> SSKQKVDLQSLPTRAYLDQTVVPILLQGLAVLAKERPPNPIEFLASYLLK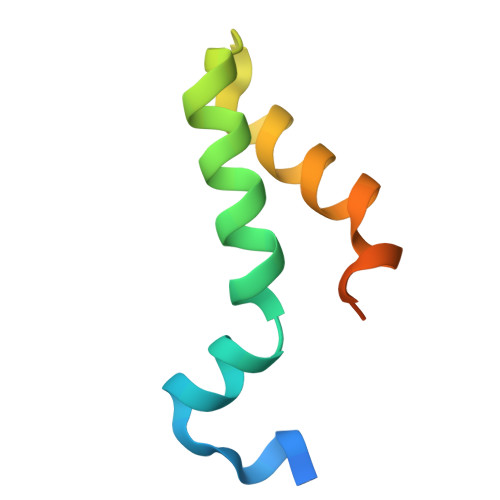NKAQFEDRNLERPHRD> MLKILWTYILFLLFISASARAEKPWYFDAIGLTETTMSLTDKNTPVVVSVVDSGVAFIGGLSDSEFAKFSFTQDGSPFPVKKSEALYIHGTAMASLIASRYGIYGVYPHALISSRRVIPDGVQDSWIRAIESIMSNVFLAPGEEKIINISGGQKGVASASVWTELLSRMGRNNDRLIVAAVGNDGADIRKLSAQQRIWPAAYHPVSSVNKKQDPVIRVAALAQYRKGETPVLHGGGITGSRFGNN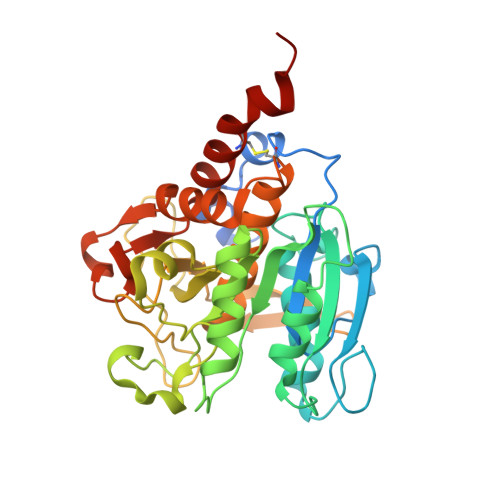WVDIAAPGQNITFLRPDAKTGTGSGTSEATAIVSGVLAAMTSCNPRATATELKRTLLESADKYPSLVDKVTEGRVLNAEKAISMFCKKNYIPVRQGRMSEEL> MKNPEEAAEGKQRIHLRPGSLRGAAPAKLHLLPCDVLVSRPAPVDRFFTPAVRHDADGLQA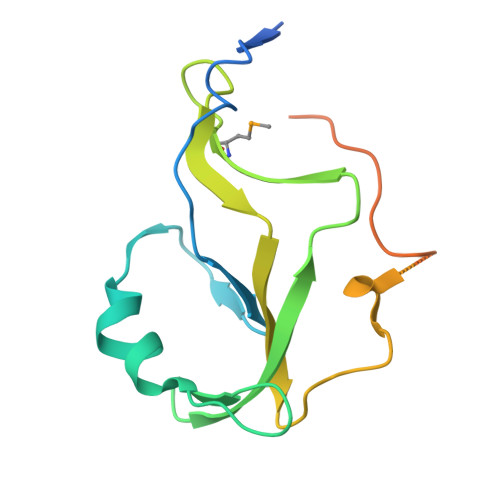SFRGRGLRGEEVAVPPGFAGFVMVTEEKGEGLIGKLNFSGDAEDKADEAQEPLERDFDRLIGATGSFSHFTLWGLETVPGPDAKVHRALGWPSLAAAIHAQVPED> SIDSALNWDGEMTVTRFDAMTGAHFVIRLDSTQLGPAAGGTRAAQYSNLADALTDAGKLAGAMTLKMAVSNLPMGGGKSVIALPAPRHSIDPSTWARILRIHAENIDKLSGNYWTGPDVNTNSADMDTLNDTTEFVFGRSLERGGAGSSAFTTAVGVFEAMKATVAHRGLGSLDGLTVLVQGLGAVGGSLASLAAEAGAQLLVADTDTERVAHAVALGHTAVALEDVLSTPCDVFAPCAMG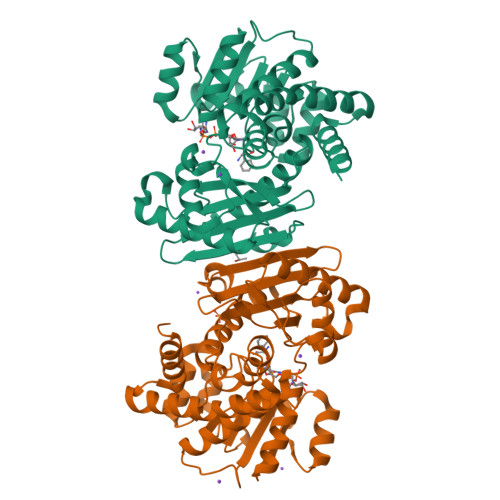GVITTEVARTLDCSVVAGAANNVIADEAASDILHARGILYAPDFVANAGGAIHLVGREVLGWSESVVHERAVAIGDTLNQVFEISDNDGVTPDEAARTLAGRRAREASTTTATA;> SIDSALNWDGEMTVTRFDSMTGAHFVIRLDSTQLGPAAGGTRAAQYSQLADALTDAGKLAGAMTLKMAVSNLPMGGGKSVIALPAPRHSIDPSTWARILRIHAENIDKLSGNYWTGPDVNTNSADMDTLNDTTEFVFGRSLERGGAGSSAFTTAVGVFEAMKATVAHRGLGSLDGLTVLVQGLGAVGGSLASLAAEAGAQLLVADTDTERVAHAVALGHTAVALEDVLSTPCDVFAPCAMGGVITTEVARTLDCSVVAGAANNVIADEAASDILHARGILYAPDFVANAGGAIHLVGREVLGWSESVVHERAVAIGDTLNQVFEISDNDGVTPDEAARTLAGRRAREASTTTATA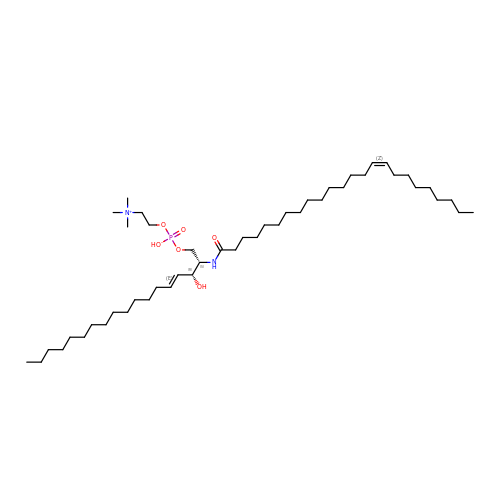sphingomyelin  | C47 H94 N2 O6 P | NHYQHBPEJLFFSO-QYKFWSDSSA-O>LKVREDENNPFYFRSSNSFQTLFENQNGRIRLLQRFNKRSPQLENLRDYRIVQFQSKPNTILLPHHADADFLLFVLSGRAILTLVNNDDRDSYNLHPGDAQRIPAGTTYYLVNPHDHQNLKMIWLAIPVNKPGRYDDFFLSSTQAQQSYLQGFSHNILETSFHSEFEEINRVLFGEEEEQRQQEGVIVELSKEQIRQLSRRAKSSSRKTISSEDEPFNLRSRNPIYSNNFGKFFEITPEKNPQLRDLDIFLSSVDINEGALLLPHFNSKAIVILVINEGDANIELVGIKEQQQKQKQEEEPLEVQRYRAELSEDDVFVIPAAYPFVVNATSNLNFLAFGINAENNQRNFLAGEKDNVVRQI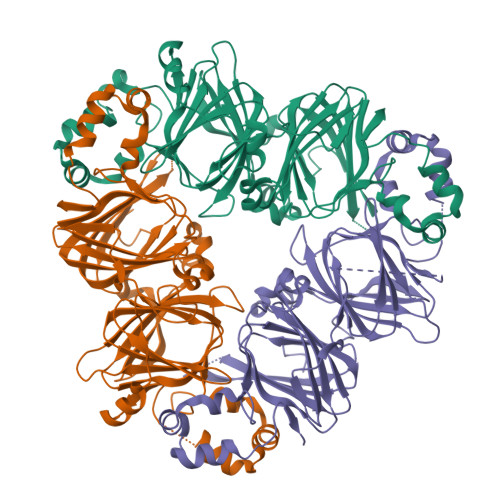ERQVQELAFPGSAQDVERLLKKQRESYFVDAQPQQKEEGSKGRKGPFPSILGALY[6x]>MQTVNNIISSVSTVESKAYRDAMSHYAGAVQIVTTAGAAGRRGLTLTAACSVSDNPPTILICLQKIHEENRIFIENGVFAINTLAGPHQQLADAFSGRIGLTQDERFELAAWEILATGAPVLKGALAAFDCRVVSVQDHS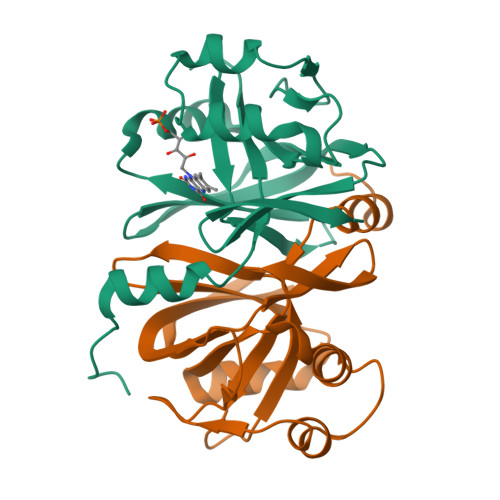THHVLFGEVVGLSSHAEEEALIYLNRRYHKLEL[4x]>MNTDRYDSLTEVEVEGLSYLYNFADGHAYHDINEHYVDIINNLQRYWQEGKDHSIPDMEKAFKNQFAELIDSSTLHSTNHFSVCPTASNSIDIVAAWLHKENKRTALIEPAFDNLYLLLKRRGVDISAFDELALKNEHQLAQIVSSGDIDALFLVNPNNPTGLEMTESEFVYLVEQCKAHNITILLDRTFRIYGKTNFDDYQILEQSGIDYVVIEDTGKTWPTQDLKISLMVYSEAISSTMRLLYEEIFLCSSNFALALLKQFVAVTAKFGVDATIKNEVRRRSETINDA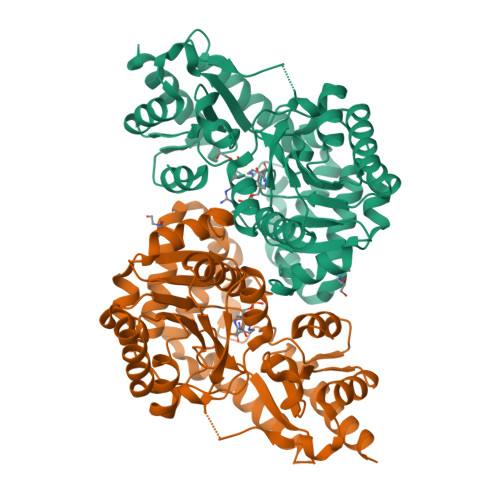LAGTGLKVFDNDEKCQLPLCWIDISATGYDDVSFAARLKEHDIAVLPGRFFYWNSKSQHTQFIRVSLMKPDAEFYEGIGKLKEAVTRILEKLEHHHHHH[4x]D-MYO INOSITOL 1,4,5,6 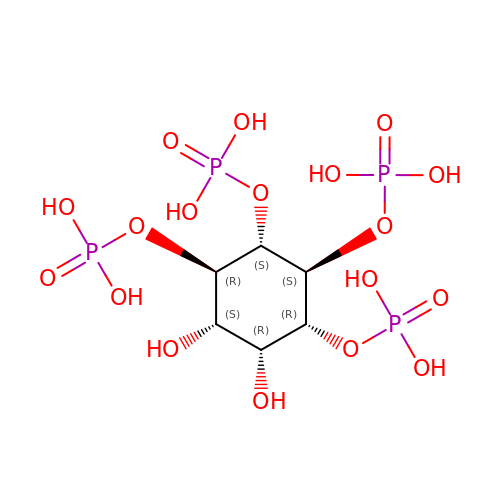TETRAKISPHOSPHATE | C6 H16 O18 P4 | MRVYFOANPDTYBY-YORTWTKJSA-N In this work, we have explored the structure and function of such non-insect OBPs in the mite Varroa destructor, a major pest of honey bee. Mass spectrometric analysis demonstrated that the six cysteines VdesOBPs, whose sequence position do not match the pattern in insect OBPs, are paired into three disulphide bridges (C1–C6, C2–C3 and C4–C5) different from that (C1–C3, C2–C5, C4–C6) of their insect counterparts. The overall folding, determined for VdesOBP1, is also novel and different from the conserved structure of insect OBPs, although some similar aspects can be recognised. Comparison with classical OBPs reveals that the second of the six α-helices found in them is lacking in VdesOBP1.

The three-dimensional structure of VdesOBP1 was solved by sulphur single-wavelength anomalous dispersion (SSAD) with a wavelength λ = 1.512 Å on beamline proxima 2A at SOLEIL synchrotron (Saint-Aubin, France). Data were collected at 1.968 Å resolution on a P3221 crystal form and a second dataset was collected at 1.81 Å resolution with wavelength λ = 0.98011 Å. VdesOBP1 crystal forms P3221 and P21 were crystallized at pH values of 7.5 and 9.5, respectively. They contain one and two molecules in the asymmetric unit, respectively. The chain was built in the electron density map of the P21 crystal form with the exception of residues 1–6 at the N-terminus, while the P3221 crystal form starts at residue 11 and lacks loop 50–53. We checked the integrity of the protein in the crystal and our analysis showed that the protein was intact, confirming that the N-terminal segment is present but not ordered in the crystal. The r.m.s.d. value between the structures of the two VdesOBP1 crystal forms is 1.55 Å. A crystallographic dimer can be reconstituted in the P3221 form, using a symmetrical molecule in the crystal packing. However, the second monomer of one form does not display the same orientation relative to that of the second form when the first monomers are superimposed. Finally, the PISA server reported an ambiguous response for the P21 form (score = 0.49) but discarded the possibility of a biological dimer in form P3221 (score = 0). All in all, it seems highly probable that the biologically relevant form is a monomer.

> APQAPASATPAKVPVIEWGKCEQLKPSESERTSKAAVVDKCLQSLPLPDPEKATQQEIDKHRESVTTCALKAEGWFDDEGVYKFDRARNEIKNKKLDSEVEEAVLLKHDACQKEATEKHDDYINQVQLYQACMDYNISQICGIKVMV>MSG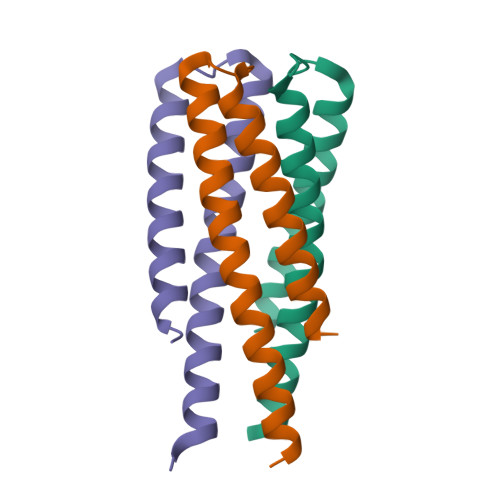KRIDEIESKLKHLEEFTTHLIKLMETMLELLKLVSDGKSDSEEYKELLEKAEEYLKQATEAAKKIGS[12x]Ferritins are ancient proteins that store iron away from the delicate machinery of the cell to be released again in a controlled fashion at the time of need. The iron storage mechanism involves binding of ferrous iron to ferritin protein followed by migration to the ferroxidase catalytic site where ferrous iron [Fe(II)] is oxidized to the ferric [Fe(III)] state. BfrB/Rv3841, the subject of this paper, is a non-heme binding ferritin. The Mtb ferritin BfrB adopts the highly conserved structural architecture of the ferritin family, consisting of 24 subunits arranged in an octahedral symmetry enclosing a hollow cavity for the storage of iron.

However, in accordance with the published genome annotation, we will continue addressing the protein as BfrB. This study describes the 3.0 Å crystal structure of Mtb BfrB. The molecular weight of BfrB being ∼20,000 Da, the Matthews constant (Vm) of 2.9 Å3/Da with solvent content of 57%, suggested 24 molecules of the protein in the asymmetric unit, corresponding to an entire 432 symmetric octahedron. The conserved region of each BfrB subunit is composed of the A-helix (H12 to S38), B-helix (P42 to D68), BC loop (R69 to R87), C-helix (P88 to D115), D-helix (F119 to R148) and E-helix (L153 to E163). In the present crystal structure of Mtb BfrB the metal site is not occupied, but the overall structure of the site is nearly identical to that of all the illustrated homologues. The residues involved in the ferroxidase centre correspond to the E22, E55 and H58 as ligands for the A-site and E99, E135 (along with E55) as ligands for the B-site. E54 in Mtb BfrB has a flipped orientation that is stabilized by formation of a salt bridge with R180 (unique to mycobacterium species) suggesting an altered C-site in Mtb BfrB. The 4-fold channel of Mtb BfrB is lined with N152, F154, E155 and R162, where the exterior mouth of the channel is negatively charged while the interior mouth is positively charged. The 3-fold channel is lined with R114, D115, E122, Q123, Q126 along with carbonyl oxygens of S171 and G172 pointing into the channel. Multiple sequence alignment revealed the presence of an extended C-terminal region comprising of 18 residues in mycobacterial ferritins. Although uncertainty existed in the side chain conformation of the Cflexible region (the proximal region of the stretch), the electron density for the Crigid (the distal region) left no ambiguity in the structural definition of this expanse.

>[24x]MTEYEGPKTKFHALMQEQIHNEFTAAQQYVAIAVYFDSEDLPQLAKHFYSQAVEERNHAMMLVQHLLDRDLRVEIPGVDTVRNQFDRPREALALALDQERTVTDQVGRLTAVARDEGDFLGEQFMQWFLQEQIEEVALMATLVRVADRAGANLFELENFVAREVDVAPAASGAPHAAGGRL Many facets of autophagy rely on the autophagy-specific ubiquitin-like protein (UBL) Atg8 in yeast (or six LC3- and GABARAP-family UBLs in higher eukaryotes, here referred to collectively as Atg8-family members) and the E1–E2–E3 enzymatic cascade that links Atg8′s C-terminus to the primary amino head group of phosphatidylethanolamine (PE) lipid molecules. The central enzyme in the Atg8 lipidation cascade is the E2, Atg313,24. Atg3 receives Atg8 from the E1 Atg7, to form a covalent, reactive Atg3~Atg8 intermediate linked by a thioester bond (referred to by ~) between the C-terminus of Atg8 and the catalytic Cys of Atg3. In addition, Atg3 displays unique, functionally important structures: an N-terminal amphipathic membrane-binding helix (N, residues 1–18); an intrinsically disordered flexible region (FR, residues 85–159); a handle region consisting of a helix and a disordered region (HR, residues 237–282) that contains an Atg8-interacting motif that is dispensable for the lipidation reaction but plays important roles in vivo; and a flexible extreme C-terminal extension (C, residues 299–310).

To illuminate roles of Atg3E123IR-binding to the Atg3cat, we determined a crystal structure lacking these interactions for comparison to the prior structure of full-length Atg3. The structure of a version of Atg3 lacking the N-terminal 18 residues and the FR region (Atg3∆NFR), determined at 2.5 Å resolution, superimposes well overall with that of full-length Atg3 (0.48 root-mean-square deviation over C-alphas). However, there are substantial differences in the catalytic Cys loop and adjacent regions. In the structure of full-length Atg3, the catalytic Cys234 is sequestered in a pocket formed by side chains from the HR and two loops. This orientation is catalytically incompetent, with the Cys distal from the structurally important Thr213 and from two other side chains (Tyr179 and His232) that are important for the lipidation reaction (right). By contrast, in the absence of the Atg3E123IR element, Atg3′s catalytic center is structurally rearranged into an activated conformation through a domino-like effect that ultimately results in remodeling a loop observed in full-length Atg3 into an additional helical turn at the N-terminus of the HR; the remodeled helix cannot restrain the side-chain from catalytic Cys234, thereby allowing the alternative orientation where Cys234 is surrounded by additional key catalytic residues (left). Moreover, it appears that the extreme C-terminal region of Atg3 also rearranges between the E123IR-bound and other states: this element undergoes a conformational change and additional C-terminal residues are visible in the crystal structure of Atg3∆NFR relative to the prior structure of full-length Atg3. In the conformation in Atg3∆NFR these residues would clash with the bound E123IR, although their nearby location also suggests potential to positively interact with the E123IR in an alternative, presently unknown conformation.

> GSKSTFLTTGQITPEEFVQAGDYLAHMFPTWKWNEESSDISYRDFLPKNKQFLIIRKVPADKRAEQAVEAKDMAQERYYDLYIAYSTSYRVPKMYIVGFNSNGSPLSPEQMFEDISADYRTKTATIEKLPFYKNSVLSVSIHPCKHANVMKILLDKVRVVRQRRRKELQEEQELDGVGDWEDLQDDIDDSLRVDQYLIVFLKFITSVTPSIQHDYTMEGW>[2x]MPNLEPAVVVPTSEAIAVDLTKLEEKLAPADSFLDRHLGPGETEQRQMLQTLGFDTLGDLIDQAVPPAIRFPRSLQLPASQSEYGAIAQLKSIASKNQVFRSYIGMGYYDTITPPVIQRNILENPGWYTAYTPYQAEIAQGRLEALLNFQTMVMDLTGLEIANASLLDEGTAAAEAMALSYGVSKSKANAFFVAQDCHPQTIEVIKTRANPLGIEVIVGDHHTFSFSTSIFGALLQYPATDGAVYDYRSFIDKAHQHQALVTLAADPLSLTLLTPPGELGADIAVGSTQRFGIPLGYGGPHAAYFATKAEYQRKMPGRIVGVSKDAHGNPALRLALQTREQHIRRDKATSNICTAQVLLAVMASMYGVYHGSTGLKNIALRIHQLTVLLAIGLKRLNYSLNNDYFFDTLRVGVGEQSAPAILKAAEGRGINLRPLVPGEVGISLDETVTVQDLLDLWQVFAGKDNLPFTPEELWSEVKTSFPADLTRQSLYLQDAVFNQYHSE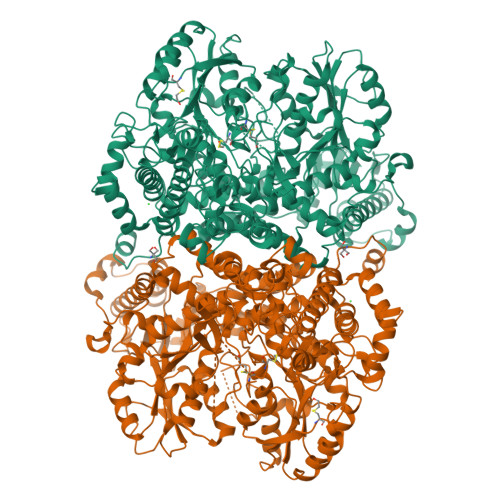TELLRYLHQLESKDLALNTSMIPLGSCTMKLNATAEMMPVTWPEFGKIHPFAPAGQTEGYQILFAQLEAWLGEITGFDAISLQPNAGSQGEYAGLQVIRQYHLSRGEEQRNICLIPESAHGTNPASAVMCGMQVVPVKCDGEGNIDVEDLTSKAEKYGDRLAALMVTYPSTHGVFEATIGTICDIVHRFGGEVYMDGANMNAQVGLCRPADFGADVCHLNLHKTFCIPHGGGGPGMGPIGVKSHLQAFLPRTSLNSTAELQAEDQSIGMISAAPYGSASILVISWMYIAMMGPQGLTKATEVAILSANYMAKRLENYYPILFRGNNELVAHECILDLRPLKKQAAIEVEDVAKRLMDFGFHAPTVSWPVLGTMMVEPTESESLGELDRFCDAMIAIYQEAQAITHGEIDPADNPLKNAPHTAQSLICGEWNHPYSQEEAAYPAPWTKQFKFWPAVGRINNTYGDRHLVCSCEGMEAYKEG> MRVLLIHADYFEYEVKDKALKNPEPISEDMKRGRMEEVLVAFISVEKVDEKNPEEVS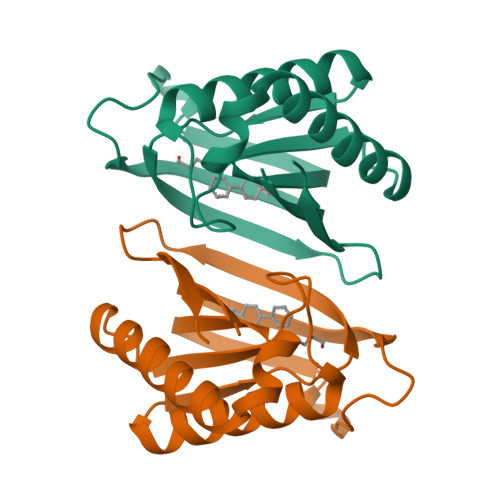LKAIEEISKVAEQVKAENVFVVPWAHLSSELAKPSVAMDILNRVYQGLKERGFNVGKAPFGYYIAAKISCKGHPLAELSRTIVPEELEHHHHHH> YDGTKCKAAGNCWEPKPGFPEKIAGSKYDPKHDPKELNKQADSIKQ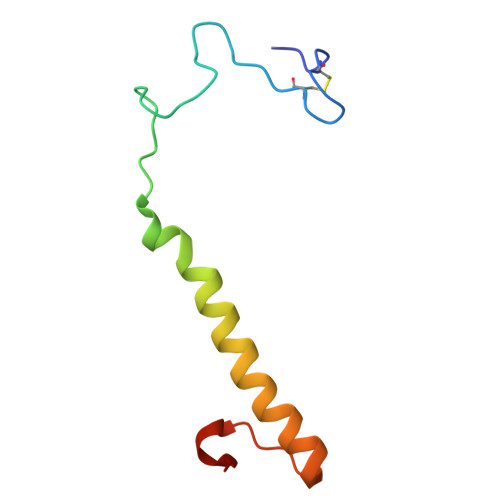MEERNKKRVENFKKTGKFEYDVAKISAN(7M)-7-[(4S)-imidazo[1,2-b]pyridazin-3-yl]-1-[(1R)-1-phenylethyl]-3-(piperazin-1-yl)pyrido[3,4-b]pyrazin-2(1H)-one 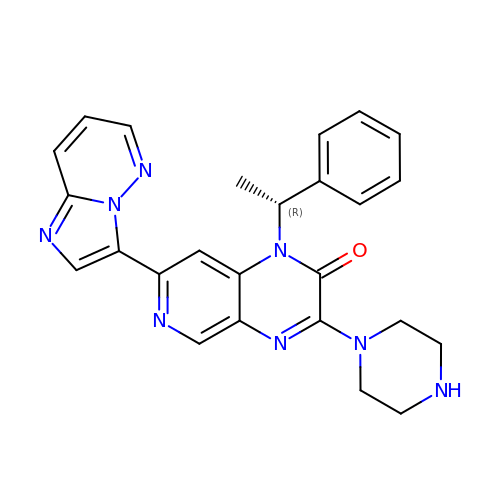| C25 H24 N8 O | JEICNGBHPARDOJ-QGZVFWFLSA-N> MSYSAYFAKAGFQFPAGLSALVAGIVALNVCTGRPTKGTKEISNAEYNATPIGYLQSPDQHPTAFPKVPGMKDVHGSPHHHH;> MMRAAQKAKQELPATVLTQTRSYLAPLRSDFTEEITAPKVASASNLVNEWNNKKQATENLMKLLQAYKDIGDAKSEPLLKNHNPRTFEDRDYP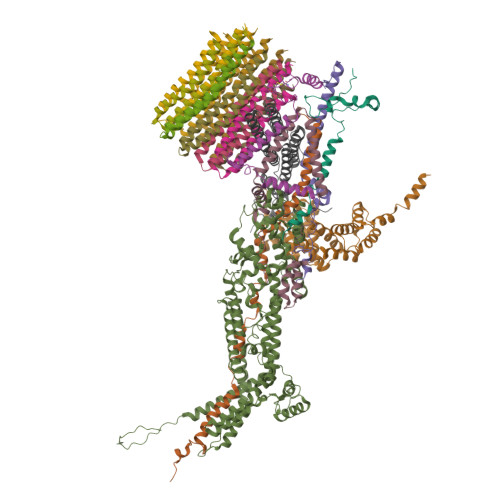VPDFRTQNLKAGDVPKFFDTVISTRASAAIASKDKFWAGRKTEAEAASAKASAAFPRVAVPEWKKGKTVSIENLNTVTDKYAAALVPKRKLALPVLPEGVKKAVEDFAASVGQAKNASEVSELLAKSLAEKAVVTEGGKVVEGFSYVSKAVAAKVIATRRAEVHERLLKLWAKRLLVSPELAIVPLNEFDAQLASKFEGISPKYQELLSAVAQGNKTFAQRLNSSPAFSSFLLKREKAESEVPPSELELEAAQKAAELEDPEVALRTLLGPQMEALGASDLLLSEQIRVITEHRYTPDRLQYKEGMKLADKIAAQEAALKEELKVIYGDNVDVKHFQASPRTPVQQLFDSLKNAAANKERAAKEAAAAASPYLAYAVTKKQEVQADPSNIPFDEVLYPQLSEELLELELSDIREDEIALEKAEEEELWLLTLTQQFKHIQKHFGIDLPHSVVAHMDPLLIKKIDWETTNALEDFDITLDDMGAEDAKEQWGAENLSHHFLPLIRYRRDLARKNGDRYGPDLVNGN;> MRQASRLALSIRQAGNVEAASAVPAMTRQFSAPGSHEHHETPLSKVMPTVVSIPRKVACLALGATKKVVCGLASSGPSQNLVSTFANKVIVEENLVNVAEIDVPFWSYWLSSAGFTSKDAFVKFAEAVKPKVAALSTSDITNLTVAFKRANYYDKDLFTGIEANVSANFTKFETEQLLQIVATFDAFNHSSVAFLDDVADSITYCNHYLAPVRAGADELATLLTYYAKNGHERADLLATVARGFSEVSLGKLSAAQRKDTVLSALKAFQTFGFYPESIEAVIGAALVSPAEYSAEELKEVEAVKVAAENALGGEFVLIQEGAHGH;> MKLLPESLQQEAATAAVVASWVLWHLDTQLLPTIMREHKLHACWAAAAKRYNEKLFKLNPSYDRVLSLPAVSKNQVLENVFHTAPKAPVEHLEKMVSANSKVYDALNLQSKRVLIWQVKPALF;> MMLRTLTRSSAVAGQAVRLFKTSAAAAEGNSVAGIIKSVNETSGANLLSSLKTIKAQAAPIYPAAASSTGYSTQAKIALFGALSWILYRADGQSKAHEWIVDLNLNVLQAAWLISFSSLIPFRAVYFAFRGMAPATASTLNGLKTFSSISL;> MVLGEVYLKDILRTPPTGAIPANVPHPFQTSFYTYATKKLIPRHWYLLGGFTFTITLYGILDGLRDSGKKKAYDEAIHAGKTPYTAGGH;> MAVTSFLGKAFEKYFYDFSAYEQFGLNRFLSSKGQYVALRHVGFVMVGVNVLLAANFPFNPPFPTIGMCPAGWEGTWVCQADKAKALEMYKEWKKSN;>[10x]MSVQRLSLGAARCLSAGVARVQASQALVAQKAVAVAPTRAQAAPAEVAQVRSMSVLAASKMVGAGCATIALAGVGAGLGVMFGSLINGAARNPNIAKQLVGYALLGFALTESIALFSLLVVFLILFA;> MSVLSSVSMGSRIGSSLLGRSSAYLAQCGFSTRSNLNGSIDTSSSVFQALSSDNENKPAASPLNVKLPGMSCSSILLPKTSRIAVPFGNQTMAMSSVRDVKTGSLPTNFLTGVYRFWRSQNPAEKPHDPVNDRLLPAVVDASDKRASIGTWATTFFCTIISCNLLGLMPFNEAPTSGLGFATGLGVSVWATATILGLSKTGFKFPGHFIPGGTPWPMAFIFVPLETISYTFRAVSLGVRLWVNMLAGHTLLHILTGMALALPFSLGFFSMVPATFGVCCLLSALVGLEYLVAVLQSGVFSILSTVYVGEFNHDKFIGPAAKIVKKIH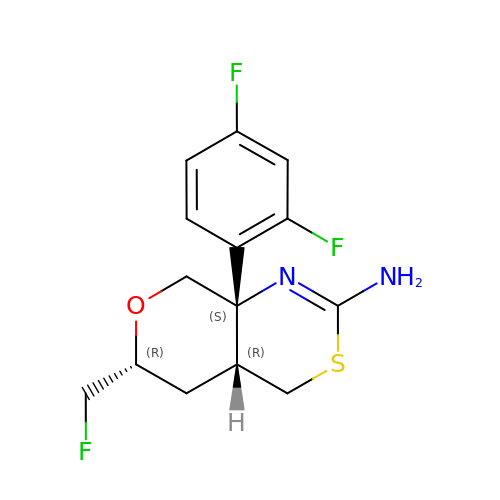(4aR,6R,8aS)-8a-(2,4-difluorophenyl)-6-(fluoromethyl)-4,4a,5,6,8,8a-hexahydropyrano[3,4-d][1,3]thiazin-2-amine | C14 H15 F3 N2 O S | HUZWRILIHNBINL-HNXYLICVSA-N>[4x]MPIMLEDYQKNFLELAIECQALRFGSFKLKSGRESPYFFNLGLFNTGKLLSNLATAYAIAIIQSDLKFDVIFG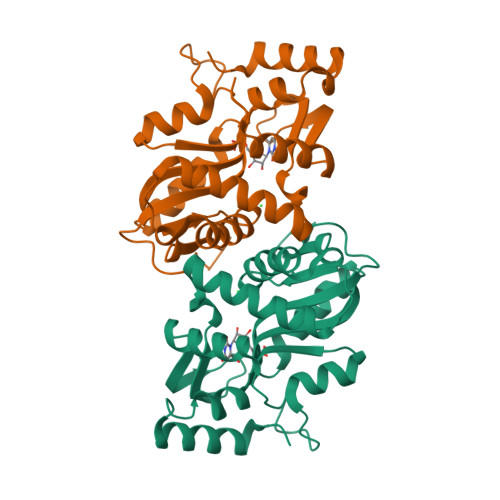PAYKGIPLAAIVCVKLAEIGGSKFQNIQYAFNRKEAKDHGEGGIIVGSALENKRILIIDDVMTAGTAINEAFEIISNAKGQVVGSIIALDRQEVVSTDDKEGLSATQTVSKKYGIPVLSIVSLIHIITYLEGRITAEEKSKIEQYLQTYGASA> MGSSHHHHHHSSGETVRFQGHMELTPDQQTLLHFIMDSYNKQRMPQEITNKILKEAFSAEENFLILTEMATNHVQVLVEFTKKLPGFQTLDHEDQIALLKGSAVEAMFLRSAEIFNKKLPSGHSDLLEARIRNSGISDEYI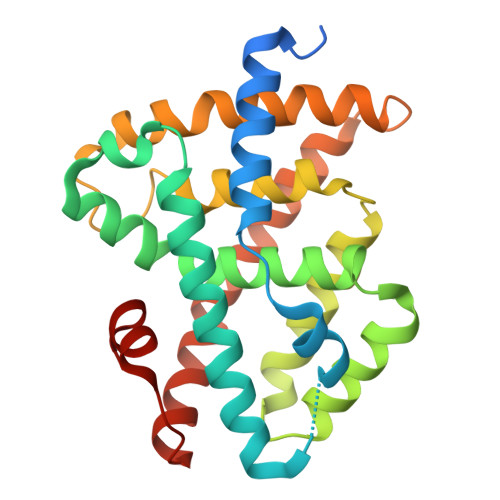TPMFSFYKSIGELKMTQEEYALLTAIVILSPDRQYIKDREAVEKLQEPLLDVLQKLCKIHQPENPQHFACLLGRLTELRTFNHHHAEMLMSWRVNDHKFTPLLCEIWDVQ>[6x]ADQKLSDFHAESGGCESCHKDGTP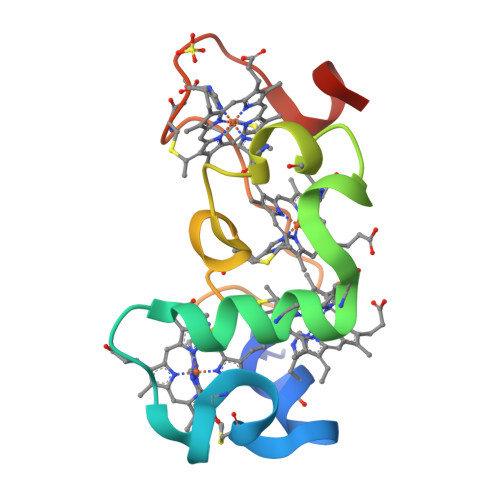SADGAFEFAQCQSCHGKLSEMDAVHKPHDGNLVCADCHAVHDMNVGQKPTCESCHDDGRTSASVLKK>[4x]GPMDLSKRFNKNLNKIEVSMIRQFDQSISDIPDVLKLTLGEPDFATPKHIKEAAKRAIDADE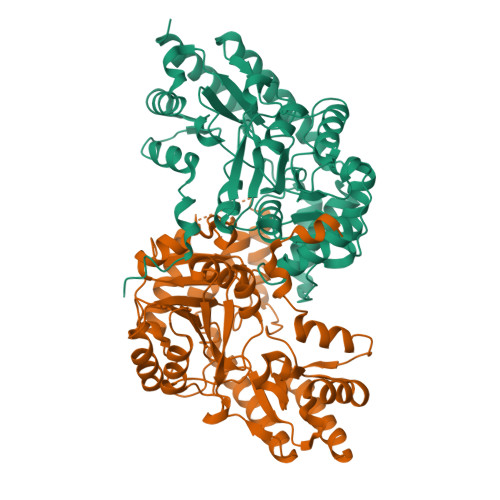SHYTGMAGLLALRQAASAFVKEKYHLTYNPDNEILVTIGATEALSASLTAILEPGDKVLLPAPAYPGYEPVVNLVGAEVVEIDTRSNDFVLTPEMLEEAILKEGEALKAVILNYPTNPTGVTYSRQQIKNLAEVLKKYPIFVISDEVYAELTYTGESHVSIAEYLPDQTILISGLSKSHAMTGWRLGLIFAPAVLTAQLIKSHQYLVTAATTSVQFAAIEALTNGKDDALPMKEEYIKRRDYIIEKMEAMKFKIIKPDGAFYIFAKIPVAQGQDSFKFLQDFAKEKAVAFIPGVAFGKYGEGYLRISYAASMETIKEAMKRLKEFMEQYAD>[8x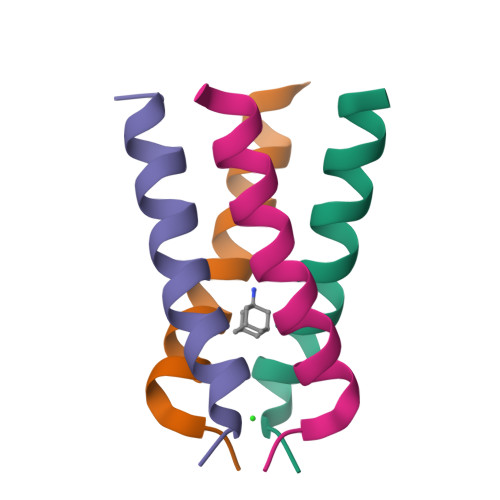]XSSDPLVVAASIIGILHLILWILDRLX> MANKTYKIGKNAGYDGCGLCLAAISENEAIKVKYLRDICPDYD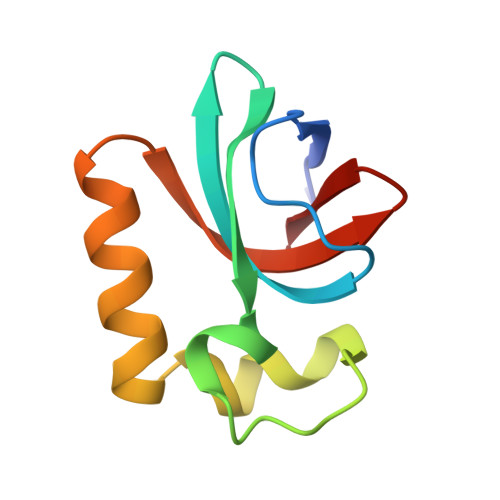GDDKAEDWLRWGTDSRVKAAALEMEQYAYTSVGMASCWEFVEL> MKTRQNVYELKDDTLSWYSRAVEEMKSRDINDPTSWWYQGAIHGYATYPSALTYWHDATGYPPSQQTVNSGFWNRCQHGTWYFLPWHRMYLFYFEEIVAKAIRDMGGPADW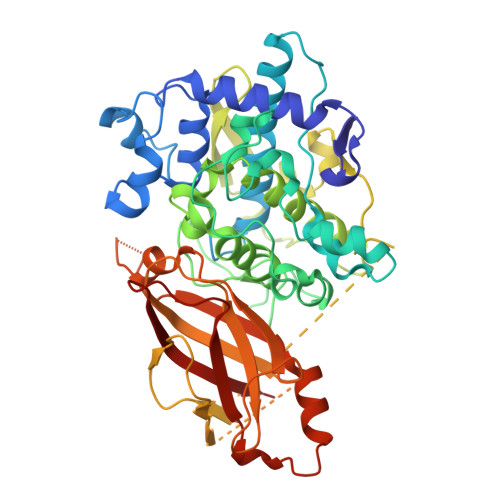TLPYWNYCEAYNTSASPSNQQQALQIPPEFGSSQGPNADFASLWIKNRRNYVLNKNNVNPWPAMNEAEFTNSGGDISFGGGVTGFAHSGGQTGQLESLPHNVVHTDINGAMGNPDTAALDPIFWLHHANIDRLWQVWLAQAGRSNPVVNAWKDFRFKFHDANGQPVEIAVKDVETTQLLGYVYTPAFPLSSTTPARRSVPAMDVVGATSASFSVGDHMAPLDLTMVPQPARGARLLAARGGDEKRTILRISNVKGKGATSPIDLFITNRDNEEGNEENFVGCIGLFGLENASTPSVESDGSGLNFAIDISDTINKLRQRDDWDEDNIRVQLIPQSKQDSDVEINVGRVSLHSEID>MSASKEVKSFLWTQSLRRELSGYCSNIKLQVVKDAQALLHGLDFSEVSNVQRLMRKQRRDDSDLKRLRDLNQAVNNLVELKSTQQKSVLRVGTLSSDDLLTLAADLEKLKSKVTRTERPLSSGVYMGNLSSQQLDQRRALLNLIGMTNGSQGSQAGRDGVVRVWDVKNAELLNNQFGTMPSLTLACLTKQGQVDLNDVVQALTDLGLIYTAKYPNTSDLDRLTQSHPILNMIDTKKSSLNISGYNFSLGAAVKAGACMLDGGNMLETIKVSPQSMDGILKSILKVKRALGMFVSDTPGERNPYENILYKICLSGDGWPYIASRTSIVGRAWENTVVDLETDGKPQKIGSGNSNKSLQSAGFSAGLTYSQLMTLKDAMLQLDPNAKTWMDIEGRPEDPVEVALYQPISGCYIHFFREPTDLKQFKQDAKYSHGIDIADLFAAQPGLTSAVIEALPRNMVIT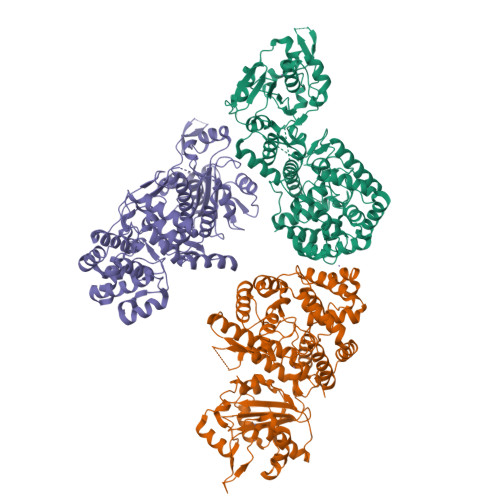CQGSEDIKKLLESQGRKDIKLIDIALSKIDSRKFENAVWDQYKDLCHMHTGVVVEKKKRGGKEEITPHCALMDCIMFDAAVSGGLNTLVLRAVLPRDMVFRTSTPRVVLDYKDHDGHHHHHH[3x]> MVGLIWAQATSGVIGRGGDIPWRLPEDQAHFREITMGHTIVMGRRVWDSLPAKVRPLPGRRNVVLSRQADFMASGAEVVGSLEEALTSPETWVIGGGQVYALALPYATRCEVTEVDIGLPREAGDALAPVLDETWRGE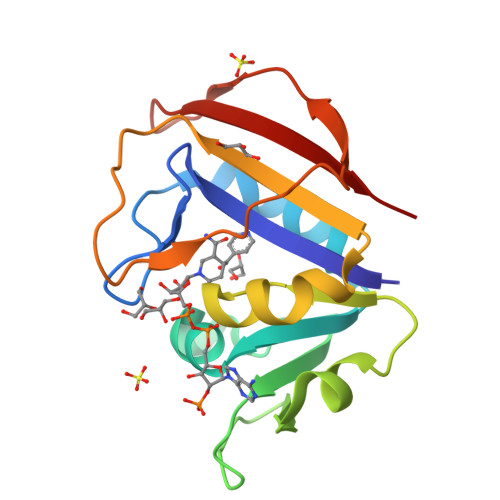TGEWRFSRSGLRYRLYSYHRS> MGKIATKYHGDIEIHEKDIVRFEQGIPGFLEEKQFVLLQLEDTPFIILQSVNTPALGFVL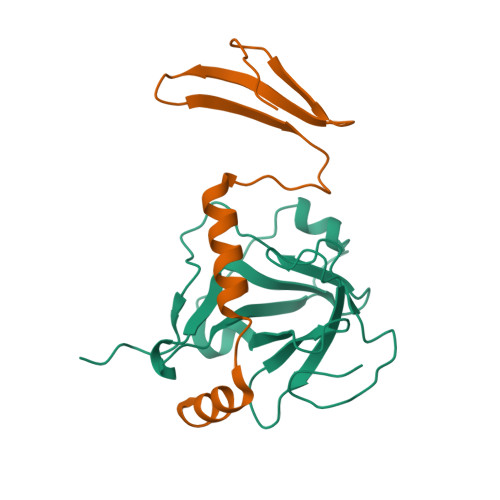IEPFSYFPTYEIDLDDNTLEQLQITGEQDVALYVILTVADPFDDTTANLQAPIVINVHKRLGKQVILTNTNYKTKHRLFPEKVAKHHHHHH;> MGLVLTRKLKEAIQIGDDIEITVLAIQGDQVKLGINAPKHVEIHRKEIYLAIQAENNAASHASKSSLKRLNEQLKHLKGGKQA>[3x]MSTAVQFRGGTTAQHATFTGAAREITVDTDKNTVVVHDGATAGGFPLARHDLVKTAFIKADKSAVAFTRTGNATASIKAGTIVEVNGKLVQFTADTAITMPALTAGTDYAIYVCDDGTVRADSNFSAPTGYTSTTARKVGGFHYAPGSNAAAQAGGNTTAQINEYSLWDIKFRPAALDPRGM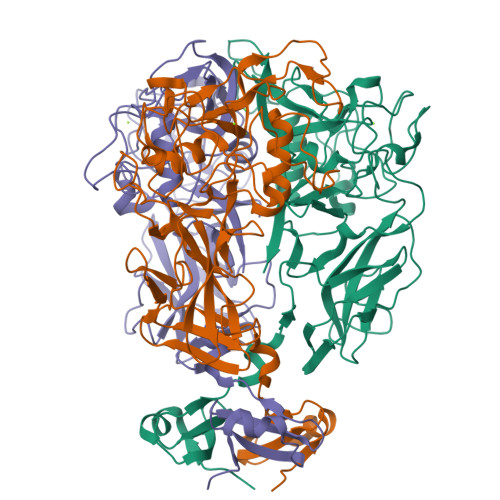TLVAGAFWADIYLLGVNHLTDGTSKYNVTIADGSASPKKSTKFGGDGSAAYSDGAWYNFAEVMTHHGKRLPNYNEFQALAFGTTEATSSGGTDVPTTGVNGTGATSAWNIFTSKWGVVQASGCLWTWGNEFGGVNGASEYTANTGGRGSVYAQPAAALFGGNWNSTSNSGSRAANWNSGPSNSPANIGARGVCDHLILE> MALMQELYSTPASRLDSFVAQWLQPHREWKEEVLDAVRTVEEFLRQEHFQGKRGLDQDVRVLKVVKVGSFGNGTVLRSTREVELVAFLSCFHSFQEAAKHHKDVLRLIWKTMWQSQDLLDLGLEDLRMEQRVPDALVFTIQTRGTAEPITVTIVPAYRALGPSLPNSQPPPEVYVSLIKACGGPGNFCPSFSELQRNFVKHRPTKLKSLLRLVKHWYQQYVKARSPRANLPPLYALELLTIYAWEMGTEEDENFMLDEGFTTVMDLLLEYEVICIYWTKYYTLHNAIIEDCVRKQLKKERPIILDPADPTLNVAEGYRWDIVAQRASQCLKQDCCYDNRENPISSWNVKRGSSHHHHHH

The 2′-5′ oligoadenylate synthetases (OASs) are a family of IFN- and virus-induced antiviral restriction factors that provide protection against a wide spectrum of RNA and DNA viruses. OASL, on the other hand, is devoid of enzymatic activity in part due to an incomplete catalytic triad in which the third carboxyl acid in position 152 has been substituted by a threonine. The 350 N-terminal residues of OASL have 39% amino acid identity with OAS1 and are known as the OAS-like domain (OLD). Recently it was discovered that the UbLD of OASL could substitute for K63-linked pUb and interact with the CARDs of RIG-I. OASL thereby enhances RIG-I signaling leading to an amplified antiviral response.

We expressed the OLD (42 kDa) in E. coli and purified it to ∼95% homogeneity by immobilized metal affinity chromatography, affinity chromatography and size exclusion chromatography. Crystallization conditions for the OLD were established using standard commercial screens and the optimized crystals diffracted to 1.6 Å. Phases were determined by molecular replacement using the structure of porcine OAS1 as a search model. However, no density was observed for the four most N-terminal residues or for the two most C-terminal residues and the C-terminal 6xHis-tag. Likewise, two loop regions spanning the residues 52–56 and 182–186 did not display well-defined electron density. The N-terminal lobe harbors the five-stranded β-sheet found in all polymerases. The C-terminal lobe is a four-helix bundle with a three-stranded mixed β-sheet with an additional interstrand α-helix connection. The crystal structure of the OLD exhibits a high similarity with active OAS1 and both proteins form the αN4 helix, which is absent in inactive OAS1. Notably, only after the binding of dsRNA does OAS1 form a rigid αN4 helix, which participates in coordinating the triphosphate of the donor ATP in 2-5A synthesis, however, in OASL the αN4 is intrinsically present. OASL intrinsically forms the αN4 helix due to residues Val67, Phe70 and Asn72 that anchor the loop and form the αN4 helix.>[4x]SKKEILLDFIEKNNGIVTNKDCKALGIP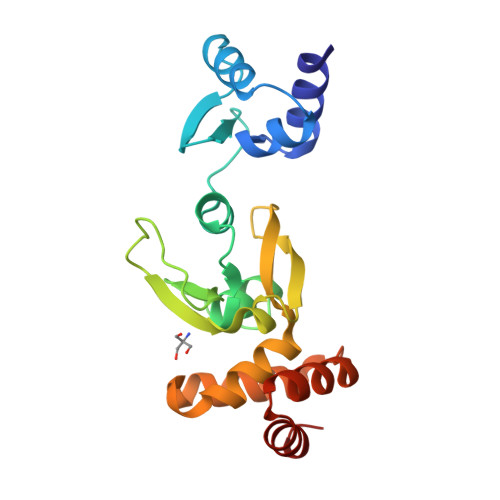TIYLTRLEKEGIIFRVEKGIFLTQNGDYDEYYFFQYRFPKAIFSYISALYLQQFTDEIPQYFDVTVPRGYRFNTPPANLNIHFVSKEYSELGMTTVPTPMGNNVRVYDFERIICDFVIHREKIDSELFVKTLQSYGNYPKKNLAKLYEYATKMNTLEKVKQTLEVLI> AFTACEKQTIGKIAQVLAKSPEAYGAECLARLFVTHPGSKSYFEYKDYSAAGAKVQVHGGKVIRAVVKAA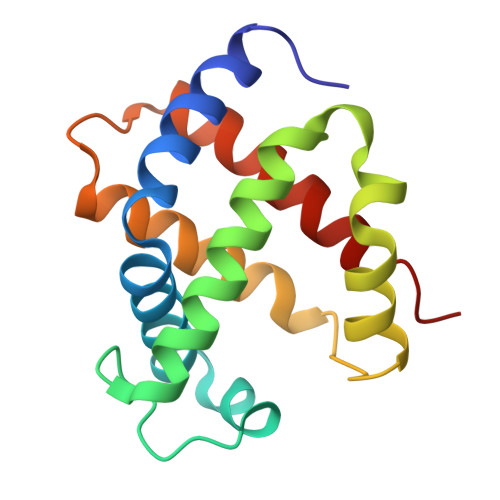EHVDDLHSHLETLALTHGKKLLVDPQNFPMLSECIIVTLATHLTEFSPDTHCAVDKLLSAICQELSSRYR> KEEKLTMTNQAKKLSRINGREFLKQSFNLQQQLLASQLNLSRTITHDGTMGEVNESYFLSIIRQYLPERYSVDRGVVVDSEGQTSDQIDAVIFDRHYTPTLLDQQGHRFIPAEAVYAVLEVKPTINKTYLEYAADKAASVRKLYRTSTVIKNIYGTAKPVEHFPIVAGIVAIDVEWQDGLGKAFTENLQAVSSDENRKLDCGLAVSGACFDSYDEEIKIRSGENALIFF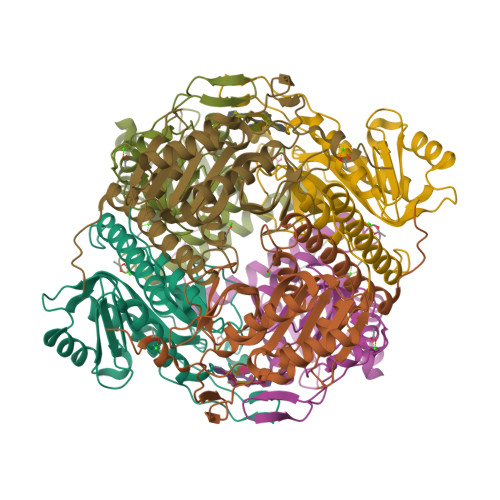LFRLLGKLQSLGTVPAIDWRVYIDSLE> ADASDWLNRLAEADRQNSFQGTFVYERNGSFSTHEIWHRVESDGAV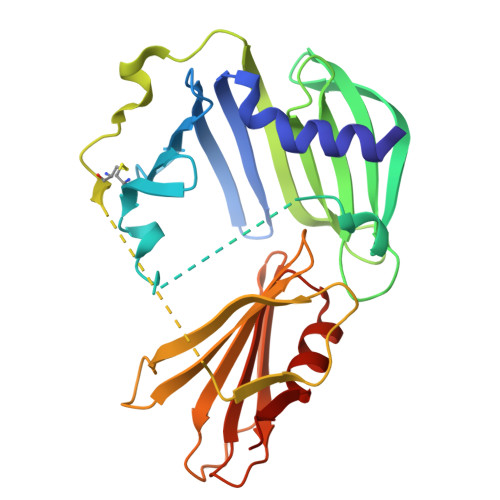RERLLQLDGARQEVVRVDGRTQCISGGLADQLADAQLWPVRKFDPSQLASWYDLRLVGESRVAGRPAVVLAVTPRDQHRYGFELHLDRDTGLPLKSLLLNEKGQLLERFQFTQLNTGAAPAEDQLQAGAECQVVGPAKADGEKTVAWRSEWLPPGFTLTRSFMRRSPVTPDPVACLTYGDGLARFSVFIEPLHGAMVGDARSQLGPTVVVSKRLQTDDGGQMVTVVGEVPLGTAERVALSIRPEAAAQK LPMOs are reducing agent- and O2-dependent copper metalloenzymes now classified as auxiliary activity families AA9–AA11 and AA137–11. Extensive spectroscopic and structural studies on LPMOs have shown that the enzyme’s active site contains a single copper ion, which is coordinated by the amino terminus nitrogen atom, by a side chain nitrogen atom of the N-terminal histidine, and by the side chain nitrogen atom of an additional histidine, in a structural motif known as the histidine brace. What is distinctive about LPMOs is that they oxidatively rather than hydrolytically cleave polysaccharides producing saccharides with oxidized ends. We report herein a study into the principal structural and electronic factors of the reactivity of two AA9 LPMOs with a range of substrates.

To understand better how protein structure might influence the similarities and differences in CvAA9A and LsAA9A substrate cleavage patterns, the X-ray crystal structure of CvAA9A was solved. The Cu-coordinating amino-acid residues are MeHis1 and His79 (with equatorial distances to the Cu ranging from 2.0 to 2.1 Å), while a non-coordinating Tyr169 occupies the axial position (2.6–2.8 Å). No exogenous ligands are evident within 3.0 Å of the Cu-ion indicating that the active site is mostly in a photoreduced Cu(I) state. A ‘pocket-water’ is bound in an H-bond network with the amide-nitrogen and oxygen of Asp76 and MeHis1, respectively. The active-site geometry of CvAA9A thus closely resembles that of LsAA9A. However, there are some amino-acid differences in CvAA9A compared to LsAA9A at subsites +2 and −1. All three of the subsite +2 substrate-binding residues in LsAA9A (Asn28, His66 and Asn67) are different in CvAA9A (Thr28, Arg67 and Val68). For example, LsAA9A’s preference to cleave Cell4 into Cell2 (as shown for NcLPMO9C18), compared to the product profile of CvAA9A of Cell3, Cell2 and Glc, could be attributed to binding cleft interactions at the +2 subsite. This is because, though CvAA9A shares the same fold, active site co-ordination and overall structure with LsAA9A, it lacks all three of the subsite +2 substrate-binding residues in LsAA9A (Asn28, His66 and Asn67). Crystals of CvAA9A were soaked with Cell3 and Cell6 oligosaccharides but this did not result in any catalytically relevant complex.

>HTRMFSVWVNGVDQGDGQNVYIRTPPNTDPIKDLASPALACNVKGGEPVPQFVSASAGDKLTFEWYRVKRGDDIIDPSHSGPITTWIAAFTSPTMDGTGPVWSKIHEEGYDASTKSWAVDKLIANKGMWDFTLPSQLKPGKYMLRQEIVAHHESDATFDKNPKRGAQFYPSCVQVDVKGVGGDAVPDQAFDFNKGYKYSDPGIAFDMYTDFDSYPIPGPPVWDAQDEGCCFIDGVDTTSVKEVVKQIICVLK[6x]3-{2,6,8-TRIOXO-9-[(2S,3R,4R)-2,3,4,5-TETRAHYDROXYPENTYL]-1,2,3,6,8,9-HEXAHYDRO-7H-PURIN-7-YL}PROPYL DIHYDROGEN PHOSPHATE | C13 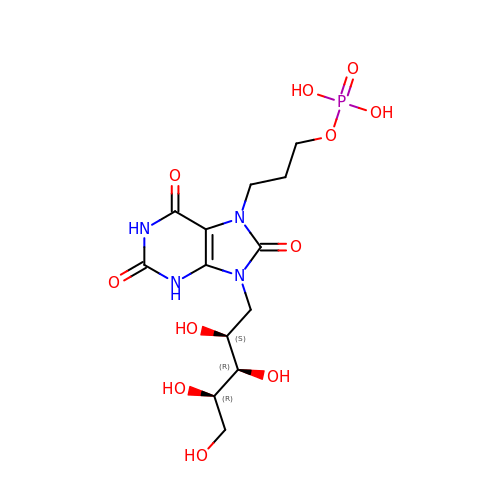H21 N4 O11 P | KPHFGOGGKPGLTM-LKEWCRSYSA-N>[2x]SHMKREEAIQNFKALLSDMVRSSDVSWSDTRRTLRKDHRWESGSLLEREEKEKLFNEHIEALTKKKREHFR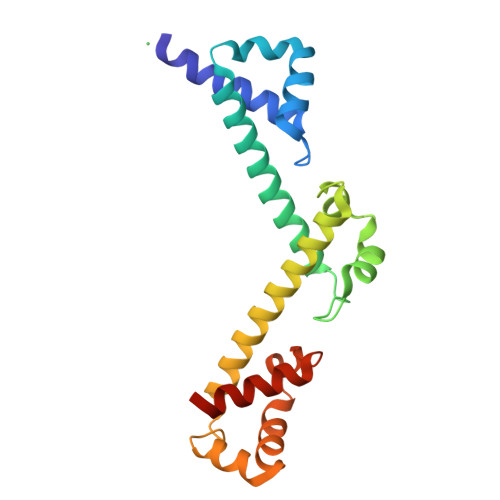QLLDETSAITLTSTWKEVKKIIKEDPRCIKFSSSDRKKQREFEEYIRDKYITAKADFRTLLKETKFITYRSKKLIQESDQHLKDVEKILQNDKRYLVLDCVPEERRKLIVAYVDDLDRR>MVLGYVSDMHTELASISQLVIAKIETIDNDILNKDIVNFIMCRSNLDNPFISFLDTVYTIIDQENYQTELINSLDDNEIIDCIVNKFMSFYKDNLENIVDAIITLKYIMNNPDFKTTYAEVLGSRI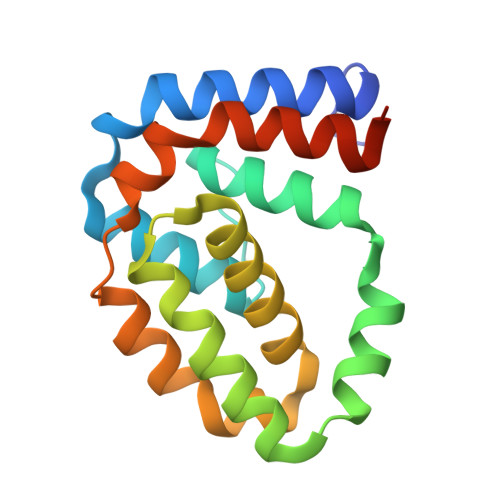ADIDIKQVIRENILQLSNDIRERYLGSKHHHHHH[2x]> MLDAQTIATVKATIPLLVETGPKLTAHFYDRMFTHNPELKEIFNMSNQRNGDQREALFNAIAAYASNIENLPALLPAVEKIAQKHTSFQIKPEQYNIVGEHLLATLDEMFSPGQEVLDAWGKAYGVLANVFINREAEIYNENASKAGGWEGTRDFRIVAKTPRSALITSFELEPVDGGAVAEYRPGQYLGVWLKPEGFPHQEIRQYSLTRKPDGKGYRIAVKREEGGQVSNWLHNHANVGDVVKLVAPAGDFFMAVADDTPVTLISAGVGQTPMLAMLDTLAKAGHTAQVNWFHAAENGDVHAFADEV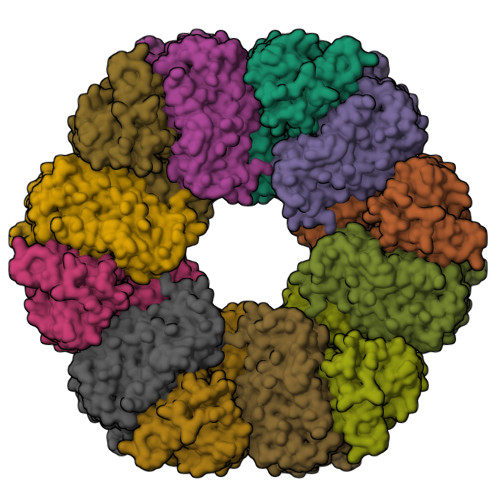KELGQSLPRFTAHTWYRQPSEADRAKGQFDSEGLMDLSKLEGAFSDPTMQFYLCGPVGFMQFTAKQLVDLGVKQENIHYECFGPHKVL>DGVGNASGDWHCDSTWSEGRVTTTSTRTWVLPTYNNHLYLRIGTTANSNTYNGFSTPWGYFDFNRFHCHFSPRDWQRLINNNWGLRPKSMRVKIFNIQVKEVTTSNGETT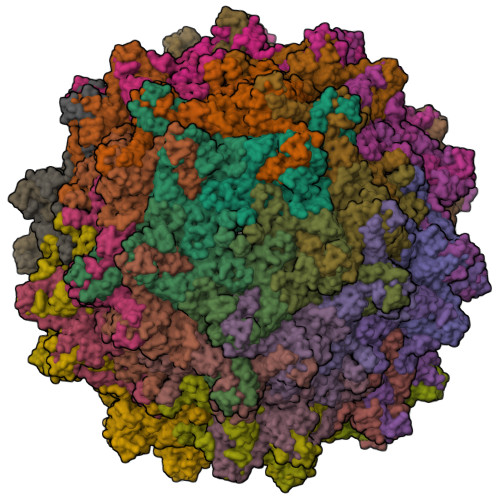VANNLTSTVQIFADSTYELPYVMDAGQEGSFPPFPNDVFMVPQYGYCGVVTGKNQNQTDRNAFYCLEYFPSQMLRTGNNFEVSYQFEKVPFHSMYAHSQSLDRMMNPLLDQYLWHLQSTTTGNSLNQGTATTTYGKITTGDFAYYRKNWLPGACIKQQKFSKNANQNYKIPASGGDALLKYDTHTTLNGRWSNMAPGPPMATAGAGDSDFSNSQLIFAGPNPSGNTTTSSNNLLFTSEEEIATTNPRDTDMFGQIADNNQNATTAPHIANLDAMGIVPGMVWQNRDIYYQGPIWAKVPHTDGHFHPSPLMGGFGLKHPPPQIFIKNTPVPANPNTTFSAARINSFLTQYSTGQVAVQIDWEIQKEHSKRWNPEVQFTSNYGTQNSMLWAPDNAGNYHELRAIGSRFLTHHL[60x]> QDGKT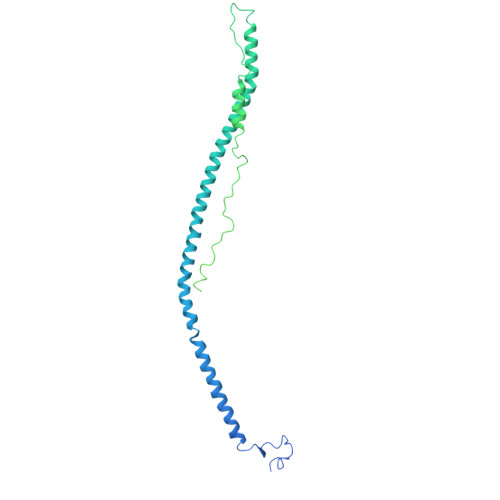TFEKEGGGGRGPRILENMHESSCKYEKNWPICVDDDWGTKCPSGCRMQGIIDDTDQNYSQRIDNIRQQLADSQNKYKTSNRVIVETINILKPGLEGAQQLDENYGHVSTELRRRIVTLKQRVATQVNRIKALQNSIQEQVVEMKRLEVDIDIKIRACKGSCARSFDYQVDKEGYDNIQKHLTQASSIDMHPDFQTTTLSTLKMRPLKDSNVPEHFKLKPSPEMQAMSAFNNIKQMQVVLERPETDHVAEARGDSSPSHTGKLITSSHRRESPSLVDKTSSASSVHRCTRTVTKKVISGPDGPREEIVEKMVSSDGSDCSHLQGGREGSTYHFSGTGDFHKLDRLLPDLESFFTHDSVSTSSRHSIGSSTSSHVTGAGSSHLGTGGKDKFTDLGEEEEDDFGGLQPSGFAAGSASHSKTVLTSSSSSFNKGGSTFETKSLKTRETSEQLGGVQHDQSAEDTPDFKARSFRPAAMSTRRSYNGKGTQK> MHYAEAATPAKSAGSAVAKKHLEAKQKIGFVHGIDGTIATIAPAASKVTVPYNTVLEIAVSATNIANALVFNLEKDGSIGVILLDNISEVRSGQDVYATGSLLKIPVGFHMLGKIINPLGKEIPTGLFTKAAPLLDDTKLGLVEEMAPNIVSRQPVNYNLLTGYKVIDTLIPVGRGQRELILGDRQTGKTSIALSTILNQTKVNNEILSKNNVLSVYVSIGQRCSNVARIHRLLTEYDAMKYCTIVAATAADPAGLQYLAPYAGTTLGEEFRNSGRHILLVYDDLSKQAVSYRQISLLLRRPPGREAYPGDVFYLHSRLLERSAMMSPQKGSGSLTSLPIVETLSNDVTAYIVTNVISITDGQIYLDAKLFTGGQRPAVNIGLSVSRVGSSAQNKAMKKVGGALKMLMGEYRKMAGEQTSGSQNVSPVMIRGARCLQLFNQKGPSYFMDAIVA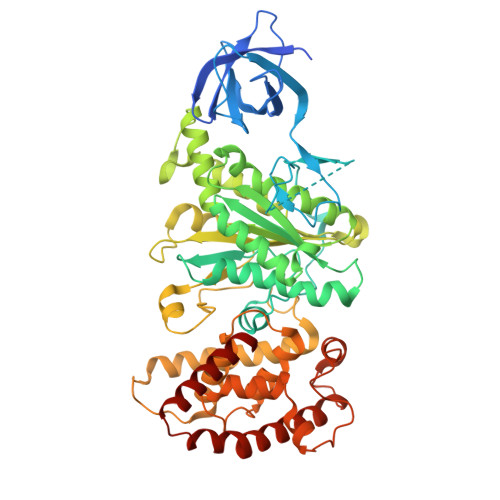LYAVTNGYMDDVKLQYSKFYEFLLLNKDLPVLYGQVNNKYFYMYNKNLNYFIRYFGLNHEILEPELKKYIEIHTNLFLDNYQSRMNELKSDEDLVQLKNLLYACKRTV Gene transfer agents (GTAs) are DNA-containing phage-like particles produced by some species of bacteria and archaea. The genes encoding proteins that form Rhodobacter capsulatus GTA particles (RcGTA) are derived from phage DNA, which has been integrated into the bacterial genome. Here, we use cryo-electron microscopy (cryo-EM) to determine the structures of RcGTA before and after DNA ejection, and to visualize the interactions of RcGTA with R. capsulatus cells. Particles of RcGTA have heads with a diameter of 38-nm and 49-nm long tails.

The structure of the RcGTA baseplate with imposed threefold symmetry has been determined to a resolution of 4.0 Å. The core of the RcGTA baseplate, formed by the hub (Rcc01696, g13) and multi-domain protein designated megatron (Rcc01698, g15) proteins, is decorated with tail fibers. The hub protein can be divided into attachment (residues 1-142), ion-binding, oligosaccharide-binding (168–249), and clip domains (264–296). The structure of the megatron protein is composed of iris/penetration (residues 1–46), adhesin-like (47–229), peripheral (230–744), central (745–984), and fiber-binding (985–1304) domains. The iris/penetration domain of the megatron protein contains α-helix 1 (residues 7–16), an extended loop, disordered region (22–37), and α-helix 2 (38–46). Helices α1 from three megatron proteins form an iris-like constriction that blocks the central channel of the RcGTA tail. Attachment of the RcGTA baseplate to the tail is enabled by the binding of the attachment domain of the hub protein and central domain of the megatron protein to the N-terminal Ala2, long loops, and C-terminal Arg209 of the distal tail proteins. The mismatch between the six-fold symmetry of the tail and threefold symmetry of the baseplate is resolved by the different conformations of residues from the long loops of odd and even subunits of distal tail proteins, which enable them to interact with hub and megatron proteins, respectively. The trimers of hub and megatron proteins form a compact complex with a buried surface area of the interaction interface of 3550 Å2. The native baseplate of RcGTA does not contain the space necessary to shift the α-helices 1 away from the pore.

>[2x]MAFHEVRFPANLSFGSVGGPERRTEIVTLSSGHEERNSPWAHSRRHYDAGVGLRSLDDVERLIAFFEARGGQLHGFRWKDWADFKSCPASRAVAHEDQLIGMGDGVTTAFQLVKTYVSGGQSYLRPIVKPVEGTVKLGIAGDHQAEAVNFAVDHATGIVSFNEPPPQGARVTAGFEFDVPVRFDTDRIAVSVQSFQAGDLPQVPVVEVRI;> MAYPESLKAHLQGGVTTLARAWALARADGRVLGFTDHDVVLRFDGISFEPGSGMTAKAVLQGTGLSVDNTESYGALSSEAITEADLLAGRYDGAAVTVWLVNWADPAMRAVIFRGHLGEVSRGAGAFTAELRGLTAALGQEQGRIYHPRCAAVLGDGRCRFDLTKDGYALEAALGGVDEAVVLRLAEGAGFEDRWFEKGRLVVLDGAAAGLIGVVKNDRLQADGSRLIELWQRLGANPVAGDRVRIEPGCDKRAGTCRLKFDNFLNFRGFPHIPGEDWMVSYPVQSGTNDGGSLFR;> MATILLSAAGAAIGGGFGGTVLGLSGAVIGRAVGATLGRVIDQRLLGSGSQSVETGRVDRLRLSSASEGEAVGRLWGRMRVAGQVIWATRFFESASVEKSGKGVPRATVTSYSYSLSLALALCEGEILRVGRVWADGSEIEVSGLNMRVYRGGEDQLPDPKIAAVEGAEAAPAYRGIAYVVLEDLQLAPFGNRVPQFTFEVVRAAQGALAEAEPDLTRGLRAVALIPGTGEYALATTPVYLATGSGVTATQGVANQNAPGGQTDLVAALERLDEELPNCGAVSLVVSWFGDDLRCGACDVKPKVASVAEEGANMPWRVAGLERAGAEEVPRLSGQSVYGGTPADAAVIEAIAALRAAGKAVTFYPFILMAQLAGNGLPDPWNPGSAQPALPWRGRITLSVAPGRAGSPDGTAAAEAQVAGFFGAASPGDSAIAGGEVVYSGPEEWSMRRFILHYAHLCQLAGGVDAFCIGTEMVALTQIRGPSNSFPAVAAFRQLAGEVKAILGPGCKIGYAADWSEYWGYAPGNGERFFHLDPLWADENIDFIGIDNYLPLSDWRDGADHADAGWGSIHALDYLRSNIEGGEYYDWFYAAPEHRAAQIRTPITDGDHDEPWIWRAKDLRNWWLNDHHERVGGLRSEVATAWVPQSKPIWFTEMGCAAIDKGTNQPNKFLDPKSSESGLPHHSDGRRDELIQMQYLRAMTGYWGEAARNPVSAVYGGPMLDMSRAHVWAWDARPWPQFPLNTALWSDGENYARGHWISGRAVAQPLASVVAEICGAAGITEIDVSGLYGLVRGYTMTGDQTGRAGLQALMLAYGFEALERDGQLVFRMRDGRVAADLAAADLALGEGEAVVETVRAAEAEIAGRVRLAYVEAEGDFEVKAVEAVFPDAAAGAAAGSELSLALTRAQAQGIVGRWLAEARVARDTARFALPPSRGHLGTGDVVRLDLPEGKRRYRIDRVEQAGLIQVEAVRVEPGIYAPADEVEDPASLRPFAAPVPVTAVFLDLPLMKGDEDPVAPHLAVTATPWPGTVAVWSSDEDAGYALNASLGTRAVIGQTLTPLFRARPGVWDRGAALRVRLASGALDSATAAKVLNGANAMAIGDGSSENWEVFQFAEAALVEGKIWDISLRLRGQLGTDALMPEVWPEGSVVVALNGAPEQILLPSAARGLARHYRIGAAVRSYDDPSFVHRIEAFAGAGLRPFSPCHLRAEPGASGWAFRWVRRTRIDGDSWQGYEVPLGETAELYLVRVLEGTAVKREVTVGEASWSYPAALQAADGIAGAFTLEVAQVSDVYGPGLAARITVGA>[6x]GA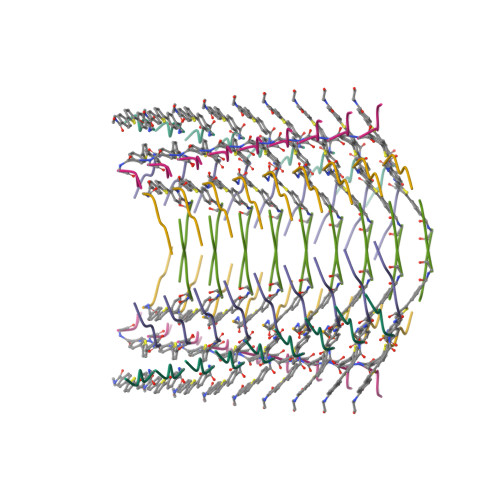VEV>[3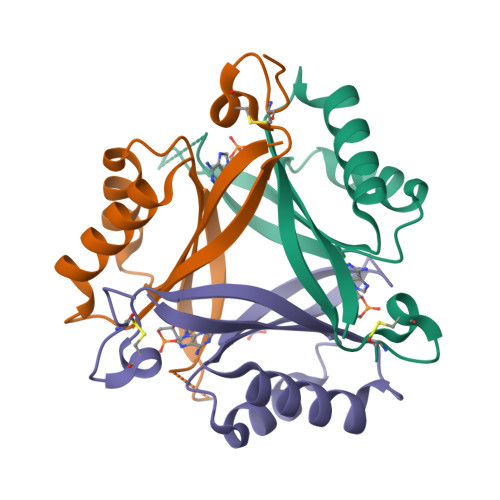x]MAKPANKLVIVTEKILLKKIAKIIDESGAKGYTVMNTGGKGSRNVRSSGQPNTSDIEANIKFEILTETREMAEEIADRVAVKYFNDYAGIIYICSAEVLYGHTFCGPEGCSAWSHPQFEK>MSFFHASQRDALNQSLAEVQGQINVSFQFFPPRTSEMEQTLWNSIDRLSSLKPKFVSVTYGANSGERDRTHSIIKGIKDRTGLEAAPHLTCIDATPDELRTIARDYWNNGIRHIVALRGDLPPGSGKPEMY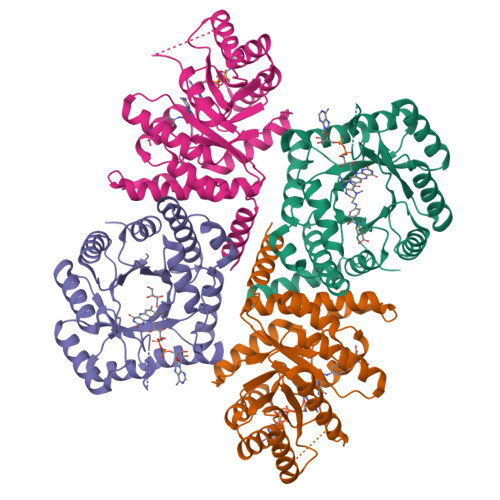ASDLVTLLKEVADFDISVAAYPEVHPEAKSAQADLLNLKRKVDAGANRAITQFFFDVESYLRFRDRCVSAGIDVEIIPGILPVSNFKQAKKLADMTNVRIPAWMAQMFDGLDDDAETRKLVGANIAMDMVKILSREGVKDFHFYTLNRAEMSYAICHTLGVRPGLLEHHHHHH[3x]>GHMSTLLINQPQYAWLKELGLREENEGVYNGSWGGRGEVITTYCPANNEPIARVRQASVADYEETVKKAREAWKIWADIPAPKRGEIVRQIGDALREKIQVLGSLVSLEMGKILVEGVGEVQEYVDICDYAVGLSRMIGGPILPSERSGHALIEQWNPVGLVGIITAFNFPVAVYGGNNAIAMICGNVCLWKGAPTTSLISVAVTKIIAKVLEDNKLPGAICSLTCGGADIGTAMAKDERVNLLSFTGSTQVGKQVGLMVQERFGRSLLELGGNNAIIAFEDADLSLVVPSALFAAVGTAGQRCTTARRLFIHESIHDEVVNRLKKAYAQIRVGNPWDPNVLYGPLHTKQAVSMFLGAVEEAKKEGGTVVYGGKVMDRPGNYVEPTIVTGLGHDASIAHTETFAPILYVFKFKNEEEVFAWNNEVKQGLSSSIFTKDLGRIFRWLGPKGSDCGIVN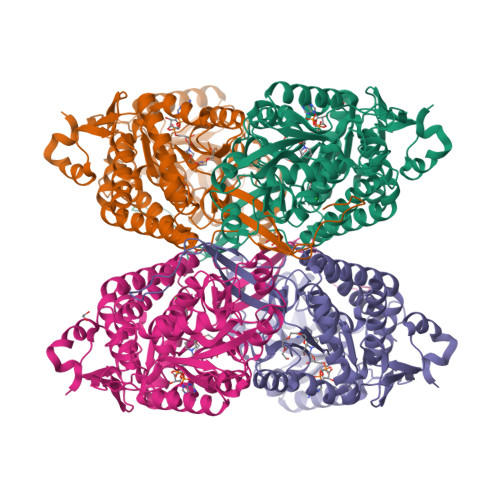VNIPTSGAEIGGAFGGEKHTGGGRESGSDAWKQYMRRSTCTINYSKDLPLAQGIKFQ[8x]>MLYIDEFKEAIDKGYILGDTVAIVRKNGK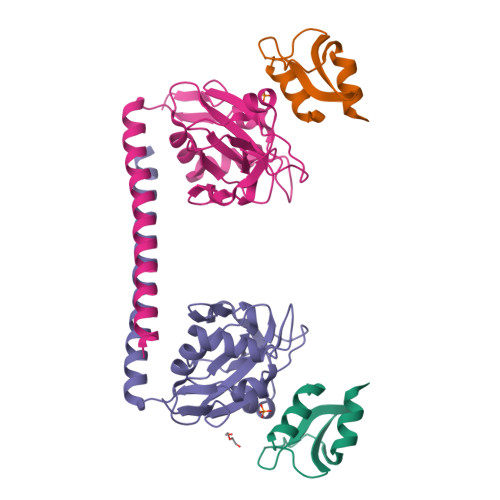IFDYVLPHEKVRDDEVVTVERVEEVMVELDKLEHHHHHH[2x];>MADSREKVTLGTVVDCFKGKAVSSKVVPGDVGLINLSDMGTLGIQYHQLRTFQMDRRQLLRYLLEDGDVLIASKGTLKKVCVFHKQNRDVVASSNITVLRPQKLLRGYYIKFFLDSPIGQALLDAADHGKDVINLSTKELLDIPIPVIPLVKQDYLINHYLRGLTDYHRKLNRAEQEWEYIQNEIQKGLGLEHHHHHH[2x]9-ethyl-8-methyl-purin-6-amine | C8 H11 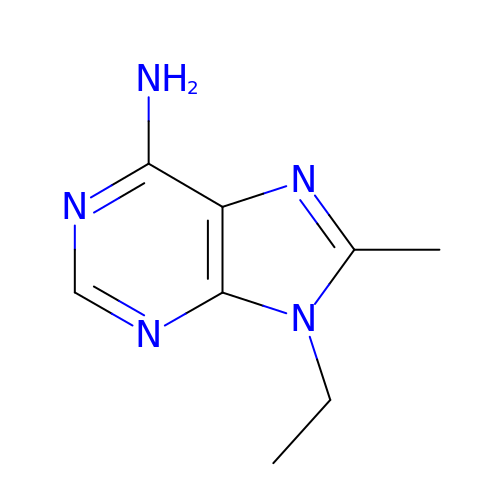N5 | XTIWXGMLCTZPOO-UHFFFAOYSA-N>[2x]MENLRQLKEKLGDKSPEDIKKLLEELETKKTTIEEERNEITQRIGELKNKI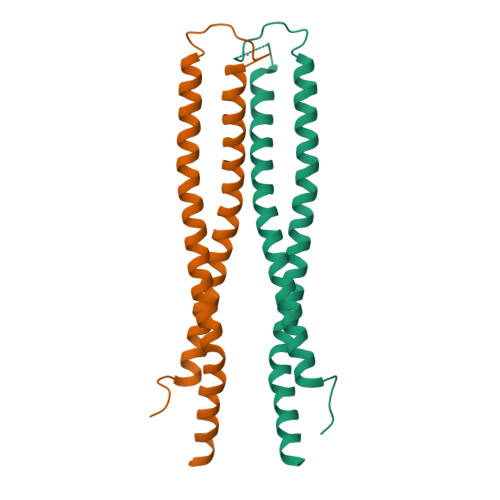GDLKTAIEELKKAKGKCPVCGRELTDEHREELLSKYHLDLNNSKNTLAKLIDRKSELERELRRIDMEIKRLTPLLTVAEQIRSIEEELN> MTTYLEFIQQNEERDGVRFSWNVWPSSRLEATRMVVPVAALFTPLKERPDLPPIQYEPVLCSRTTCRAVLNPLCQVDYRAKLWACNFCYQRNQFPPSYAGISELNQPAELLPQFSSIEYVVLRGPQMPLIFLYVVDTCMEDEDLQALKESMQMSLSLLPPTALVGLITFGRMVQVHELGCEGISKSYVFRGTKDLSAKQLQEMLGLSKVPLTQATRGPQVQQPPPSNRFLQPVQKIDMNLTDLLGELQRDPWPVPQGKRPLRSSGVALSIAVGLLECTFPNTGARIMMFIGGPATQGPGMVVGDELKTPIRSWHDIDKDNAKYVKKGTKHFEALANRAATTGHVIDIYACALDQTGLLEMKCCPNLTGGYMVMGDSFNTSLFKQTFQRVFTKDMHGQFKMGFGGTLEIKTSREIKISGAIGPCVSLNSKGPCVSENEIGTGGTCQWKICGLSPTTTLAIYFEVVNQHNAPIPQGGRGAIQFVTQYQHSSGQRRIRVTTIARNWADAQTQIQNIAASFDQEAAAILMARLAIYRAETEEGPDVLRWLDRQLIRLCQKFGEYHKDDPSSFRFSETFSLYPQFMFHLRRSSFLQVFNNSPDESSYYRHHFMRQDLTQSLIMIQPILYAYSFSGPPEPVLLDSSSILADRILLMDTFFQILIYHGETIAQWRKSGYQDMPEYENFRHLLQAPVDDAQEILHSRFPMPRYIDTEHGGSQARFLLSKVNPSQTHNNMYAWGQESGAPILTDDVSLQVFMDHLKKLAVSSA;> EGLRVVNLLQERNMLPSTPLKPPVPNLHEDIQKLNCNPELFRCTLTSIPQTQALLNKAKLPLGLLLHPFKDLVQLPVVTSSTIVRCRSCRTYINPFVSFLDQRRWKCNLCYRVNDVPEEFLYNPLTRVYGEPHRRPEVQNATIEFMAPSEYMLRPPQPPVYLFVFDVSHNAVETGYLNSVCQSLLDNLDLLPGNTRTKIGFITFDSTIHFYGLQESLSQPQMLIVSDIEDVFIPMPENLLVNLNESKELVQDLLKTLPQMFTKTLETQSALGPALQAAFKLMSPTGGRMSVFQTQLPTLGVGALKPREEPNHRSSAKDIHMTPSTDFYKKLALDCSGQQVAVDLFLLSGQYSDLASLGCISRYSAGSVYYYPSYHHQHNPVQVQKLQKELQRYLTRKIGFEAVMRIRCTKGLSIHTFHGNFFVRSTDLLSLPNVNPDAGYAVQMSVEESLTDTQLVSFQSALLYTSSKGERRIRVHTLCLPVVSTLNDVFLGADVQAISGLLANMAVDRSMTASLSDARDALVNAVIDSLSAYRSSVLSNQQPGLMVPFSLRLFPLFVLALLKQKSFQTGTNARLDERIFAMCQVKNQPLVYLMLTTHPSLYRVDNLSDEGALNISDRTIPQPPILQLSVEKLSRDGAFLMDAGSVLMLWVGKNCTQNFLSQVLGVQNYASIPQPMTDLPELDTPESARIIAFISWLR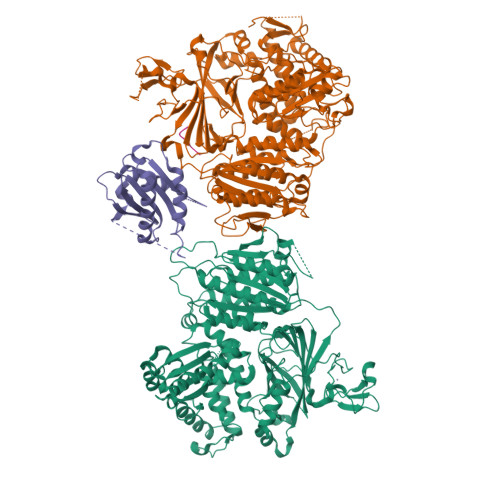EQRPFFPILYVIADESPMKANFLQNMIEDRTESALSYYEFLLHIQQQVNK;> MVLLTMIARVADGLPLAASMQEDEQSGRDLQQYQSQAKQLFRKLNEQSPTRCTLEAGAMTFHYIIEQGVCYLVLCEAAFPKKLAFAYLEDLHSEFDEQHGKKVPTVSRPYSFIEFDTFIQKTKKLYIDSRARRNLGSINTELQDVQRIMVANIEEVL;> VTSVV> IIDGAPCARGSHPWQVALLSGNQLHCGGVLVNERWVLTAAHCKMNEYTVHLGSDTLGD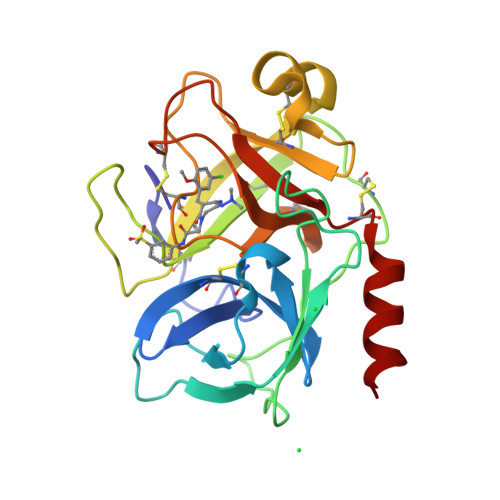RRAQRIKASKSFRHPGYSTQTHVNDLMLVKLNSQARLSSMVKKVRLPSRCEPPGTTCTVSGWGTTTSPDVTFPSDLMCVDVKLISPQDCTKVYKDLLENSMLCAGIPDSKKNACNGDSGGPLVCRGTLQGLVSWGTFPCGQPNDPGVYTQVCKFTKWINDTMKKHR> GSFTMEPLKVEKFATANRGNGLRAVTPLRPGELLFRSDPLAYTVCKGSRGVVCDRCLLGKEKLMRCSQCRVAKYCSAKCQKKAWPDHKRECKCLKSCKPRYPPDSVRLLGRVVFKLMDGAPSESEKLYSFYDLESNINKLTEDKKEGLRQLVMTFQHFMREEIQDASQLPPAFD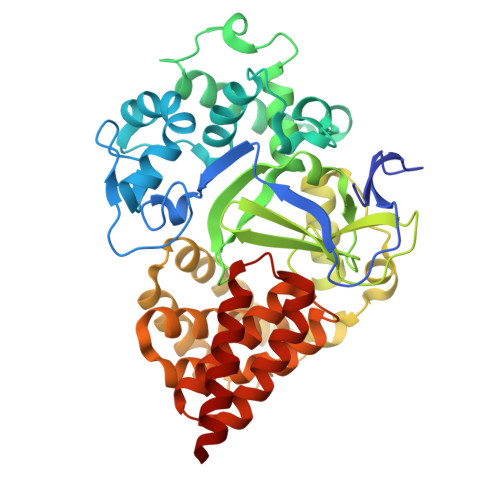LFEAFAKVICNSFTICNAEMQEVGVGLYPSISLLNHSCDPNCSIVFNGPHLLLRAVRDIEVGEELTICYLDMLMTSEERRKQLRDQYCFECDCFRCQTQDKDADMLTGDEQVWKEVQESLKKIEELKAHWKWEQVLAMCQAIISSNSERLPDINIYQLKVLDCAMDACINLGLLEEALFYGTRTMEPYRIFFPGSHPVRGVQVMKVGKLQLHQGMFPQAMKNLRLAFDIMRVTHGREHSLIEDLILLLEECDANIRAS The replication of positive-strand RNA viruses relies on virally encoded RNA-dependent RNA polymerases (RdRPs) that are capable of rapid and processive synthesis of the 7–14 kilobase viral genomes. To examine this in further detail and to validate the polymerase–RNA interactions seen in the initial poliovirus EC structures, we here present nine new coxsackievirus, rhinovirus, and poliovirus elongation complex structures at resolutions ranging from 2.1 to 2.9 Å. All the complexes feature an upstream RNA duplex that is pinched between the pinky finger and thumb domains such that the RNA exit channel is opened by ≈4 Å as compared to the polymerase alone structures. All of the complexes show the open conformation for the active site wherein the β-strands of motifs A and C are not hydrogen bonded together to fully form the RMM-fold that is commonly utilized by polymerase active sites.

Expanding on the r2 construct, the length of the upstream RNA duplex between the two ECs was shortened from 26 to 24 (r3) and 22 (r4) base pairs, and both these RNAs resulted in poliovirus EC crystals that diffracted to 2.4 Å (PV_r3) and 2.8 Å (PV_r4) resolution.

>[2x]GEIQWMRPSKEVGYPIINAPSKTKLEPSAFHYVFEGVKEPAVLTKNDPRLKTDFEEAIFSKYVGNKITEVDEYMKEAVDHYAGQLMSLDINTEQMCLEDAMYGTDGLEALDLSTSAGYPYVAMGKKKRDILNKQTRDTKEMQKLLDTYGINLPLVTYVKDELRSKTKVEQGKSRLIEASSLNDSVAMRMAFGNLYAAFHKNPGVITGSAVGCDPDLFWSKIPVLMEEKLFAFDYTGYDASLSPAWFEALKMVLEKIGFGDRVDYIDYLNHSHHLYKNKTYCVKGGMPSGCSGTSIFNSMINNLIIRTLLLKTYKGIDLDHLKMIAYGDDVIASYPHEVDASLLAQSGKDYGLTMTPADKSATFETVTWENVTFLKRFFRADEKYPFLIHPVMPMKEIHESIRWTKDPRNTQDHVRSLCLLAWHNGEEEYNKFLAKIRSVPIGRALDLPEYSTLYRRWLDSFGSSSHHHHHH> MGSSHHHHHHSSGRENLYFQGSGSNTEEEIRMELSPDLISACLALEKYLDNPNALTERELKVAY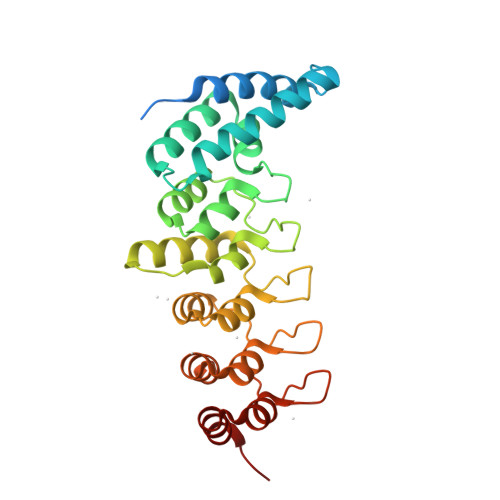TTVLQEWLRLACRSDAHPELVRRHLVTFRAMSARLLDYVVNIADSNGNTALHYSVSHANFPVVQQLLDSGVCKVDKQNRAGYSPIMLTALATLKTQDDIETVLQLFRLGNINAKASQAGQTALMLAVSHGRVDVVKALLACEADVNVQDDDGSTALMCACEHGHKEIAGLLLAVPSCDISLTDRDGSTALMVALDAGQSEIASMLYSRMNIK>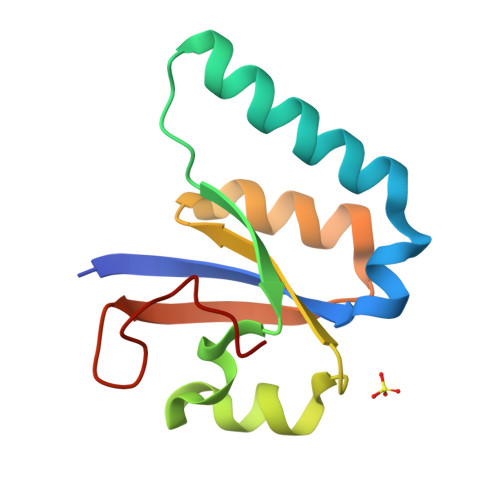 GSHMATYYYALASQKFLLEEEPFEEVLKERRRDYGEKNKEIDFWQVIQPAFLNAPELAEAKAKAPEKNVAIVSTNKSFIVWVKLRLEYVLTGEFEAPSDAIPDPLASLD PNP is a ubiquitous enzyme that reversibly converts purine nucleosides into nucleobases and α-pentose-1-phosphate, and is responsible for the regulation of nucleoside concentration within cells. The hexameric molecule of PNP from E. coli can be described as a trimer of dimers. The key role in the catalysis of natural enzyme substrates is played by Asp204, which is protonated, and by Arg217. Closing of the active site is a necessary step in catalysis; it brings Arg217 closer to Asp204 and enables the formation of a hydrogen bond between these residues, with deprotonation of Asp204 and protonation of N7 of the purine ring, which initiates catalysis.

Mutation of Asp into Asn is a substitution of one polar amino acid with another polar amino acid having different properties, namely different pKa for protonation. This mutation still allows for the formation of a hydrogen bond between a ligand and the protein, but proton transfer from the enzyme molecule to the purine ring of a substrate is impossible; thus, this mutation gives insight into the mechanism of catalysis. When the mutant D204N-PNP with Asp204 replaced by Asn204 was chosen as a catalyst, the obtained data for N2,3-ε2APu was similar to the WT PNP (Km = 12 μM, Vmax(rel) = 30). In the WT PNP-N2,3-ε2APu and D204N-PNP-N2,3-ε2APu structures, the ligand is bound in all subunits, as the electron density in the appropriate region of the active site is in this case unambiguous. In both structures, there is one subunit in the closed (chain A) and two subunits in the open (chains B and C) active site conformations; thus, an active hexamer is composed of two asymmetric open–closed dimers (A-C, A’-C’) and one symmetric open–open dimer (B-B’). In all active sites, a phosphate ion (or a sulfate ion from the crystallization liquid) is bound in a typical position, at a hydrogen bond distance from Arg43* (from the neighboring subunit) and Arg87, while in the active sites with the closed conformation, also from Arg24. In the case of the D204N enzyme, small electron density blobs observed in this part of the active site were modeled with a few water molecules. The orientation of N2,3-ε2APu in the active site cannot be determined unambiguously as, at this resolution, the electron density blob is symmetric. In the case of the WT PNP, the orientation differs in the closed and open active site conformations, whereas in the structure of the D204N enzyme, the orientation is identical in all active sites. In the case of the D204N-PNP-N2,3-ε2APu complex, the orientation of the ligand in all subunits, regardless of the active site conformation, is like in the closed active site of the WT PNP, thus pointing to the ribosylation site either at N7 or N2.

>MATPHINAEMGDFADVVLMPGDPLRAKYIAETFLEDAREVNNVRGMLGFTGTYKGRKISVMGHGMGIPSCSIYTKELITDFGVKKIIRVGSCGAVLPHVKLRDVVIGMGACTDSKVNRIRFKDHDFAAIADFDMVRNAVDAAKALGIDARVGNLFSADLFYSPDGEMFDVMEKYGILGVEMEAAGIYGVAAEFGAKALTICTVSNHIRTHEQTTAAERQTTFNDMIKIALESVLLGDKE[3x]>GEFNTIQQLMMILNSASDQPSENLISYFNNCTVNPKESILKRVKDIGYIFKEKFAKAVGQGCVEIGSQRYKLGVRLYYRVMESMLKSEEERLSIQNFSKLLNDNIFHMSLLACALEVVMATYSRSTSQNLDSGTDLSFPWILNVLNLKAFDFYKVIKSFIKAEGNLTREMIKHLERCEHRIMESLAWLSDSPLFDLIKQSKDREGPTDHLESACPLNLPLQNNHTAADMYLEPVRAPKKKSTSLSLFYKKVYRLAYLRLNTLCERLLSEHPELEHIIWTLFQHTLQNEYELMRDRHLDQIMMCSMYGICKVKNIDLKFKIIVTAYKDLPHAVQETFKRVLIKEEEYDSIIVFYNSVFMQRLKTNILQYASTRPPTLAPIPHI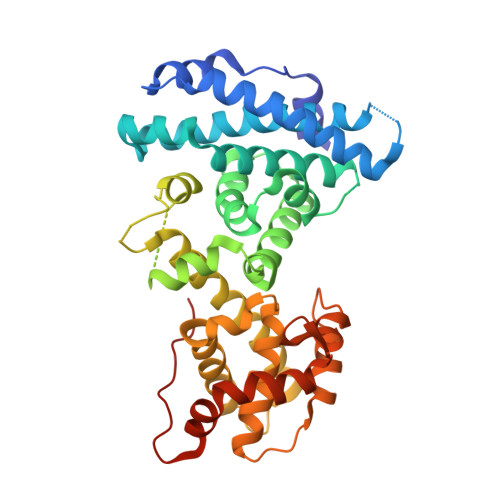PFMQRLKT[2x]> APTSSIEIVLDKTTASVGEIVTASINIKNITNFSGCQLNMKYDPAVLQPVTSSGVAYTKSTMPGAGTILNS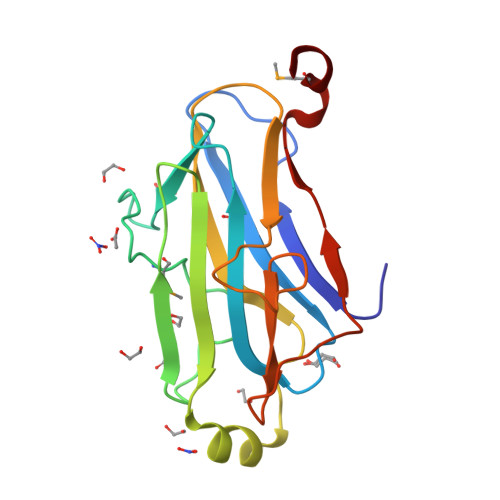DFNLRQVADNDLEKGILNFSKAYVSLDDYRTAAAPEQTGTVAVVKFKVLKEETSSISFEDTTSVPNAIDGTVLFDWNGDRIQSGYSVIQPAVINLDMIKAS> MVEATAQETDRPRFSFSIAAREGKARTGTIE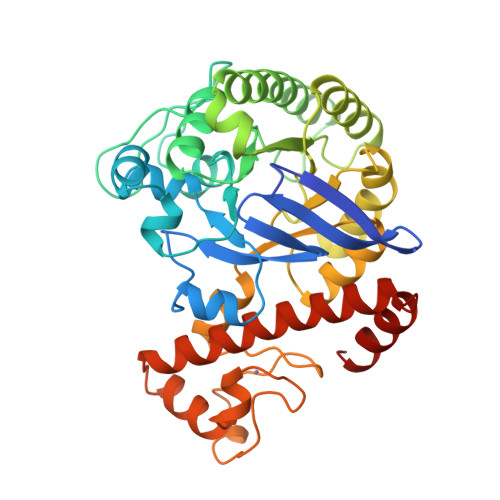MKRGVIRTPAFMPVGTAATVKALKPETVRATGADIILGNTYHLMLRPGAERIAKLGGLHSFMGWDRPILTDSGGYQVMSLSSLTKQSEEGVTFKSHLDGSRHMLSPERSIEIQHLLGSDIVMAFAECTPYPATPSRAASSMERSMRWAKRSRDAFDSRKEQAENAALFGIQQGSVFENLRQQSADALAEIGFDGYAVGGLAVGEGQDEMFRVLDFSVPMLPDDKPHYLMGVGKPDDIVGAVERGIDMFDCVLPTRSGRNGQAFTWDGPINIRNARFSEDLKPLDSECHCAVCQKWSRAYIHHLIRAGEILGAMLMTEHNIAFYQQLMQKIRDSISEGRFSQFAQDFRARYFARNS> GPGTHYGTQQIPPAYKDLAEPWIQVFGMELVGCLFSRNWNVREMALRRLSHDVSGALLLANGESTGNSGGSSGSSPSGGA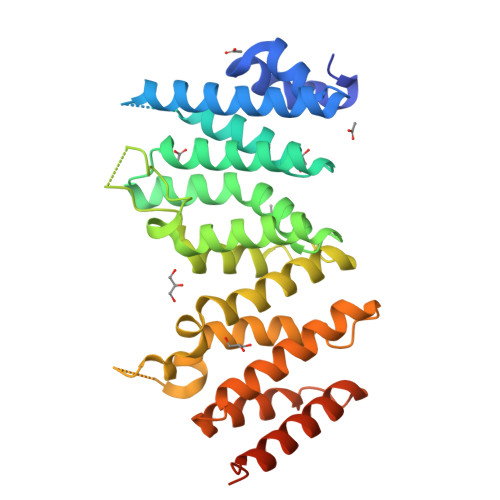TSGSSQTSISGDVVEACCSVLSMVCADPVYKVYVAALKTLRAMLVYTPCHSLAERIKLQRLLQPVVDTILVKCADANSRTSQLSISTLLELCKGQAGELAVGREILKAGSIGIGGVDYVLNCILGNQTESNNWQELLGRLCLIDRLLLEFPAEFYPHIVSTDVSQAEPVEIRYKKLLSLLTFALQSIDNSHSMVGKLSRRIYLSSARMVTTVPHVFSKLLEMLSVSSSTHFTRMRRRLMAIADEVEIAEAIQLGVEDTLDGQQDSFLQAS>MSQSGEDLHSPTYLSWRKLQLSRAKLKASSKTSALLSGFAMVAMVEVQLDHDTNVPPGMLIAFAICTTLLVAVHMLALMISTCILPNIETVSNLHSISLVHESPHERLHWYIETAWAFSTLLGLILFLLEIAILCWVKFYDLSPPAAWSATVVLIPVMIIFMAFAIHFYRSLVSHKYEVTVSGIRELEMLKEQMEQDHLEHHNNIRNNGEGEEF[24x]

Orai was identified as the protein that forms the channel’s pore and STIM was identified as its regulator. The channel is activated by the depletion of Ca2+ from the endoplasmic reticulum (ER), and as such it was characterized as the calcium release-activated calcium (CRAC) channel responsible for store-operated calcium entry (SOCE) before the molecular components were known. The channel is formed from an assembly of six Orai subunits that surround a single ion pore, which is perpendicular to the plasma membrane in a cellular setting. Each Orai subunit contains four transmembrane helices (M1-M4) and a cytosolic M4-ext helix.

To exclude the possibility that the crystal contacts in the H206A Oraicryst structure were responsible for the conformational changes we observed in the pore, we determined the structures of wild-type (WT) Oraicryst and K163W Oraicryst grown in the same crystal form (I41). Well-defined electron density maps of WT and K163W Oraicryst were obtained using non-crystallographic symmetry averaging of modest (6.9 and 6.1 Å, respectively) resolution diffraction data in the same manner as for the H206A Oraicryst structure. Anomalous-difference electron density peaks for sulfur atoms of methionine and cysteine residues in WT Oraicryst confirm the accuracy of the atomic model. The structures of WT and K163W Oraicryst reveal an ‘unlatched-closed’ conformation of the channel that resembles a hybrid of the quiescent and open conformations: the ion pores are closed as in the quiescent conformation but the M4/M4-ext regions have conformations like those observed in the H206A Oraicryst structure. The conformation of the M1-M4a portion of the channel, however, is like the quiescent conformation, and as such, the pores of WT and K163W Oraicryst are closed and indistinguishable from the pore in the structure of the quiescent conformation. The unlatched-closed conformation has analogous straightenings of M4/M4-ext as the open structure, and analogous crystal packing. Therefore, contacts within the crystal and the straightening of M4/M4-ext are not responsible for the opening of the pore that is observed with H206A Oraicryst. As in the quiescent conformation, anomalous difference electron density for an iron complex is observed in the basic region of the pore in the unlatched-closed conformation. The density is positioned roughly in the center of the basic region in the structure of WT Oraicryst and located in the lower portion of it in the structures of the K163W mutant, which removes the top ring of basic residues from the pore. Thus, while necessary, unlatching is not sufficient to open the pore.> PAPSID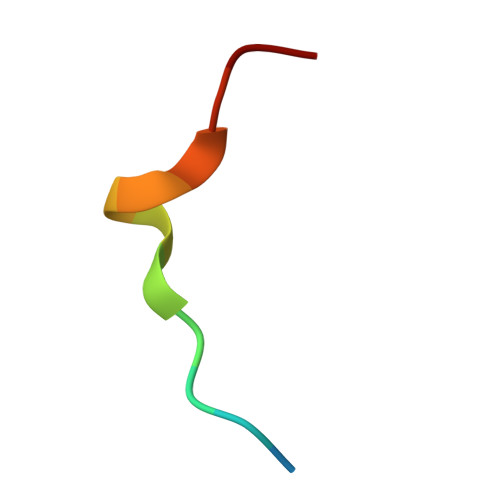RSTKPPL Type VIIb secretion systems (T7SSb) were recently proposed to mediate different aspects of Firmicutes physiology, including bacterial pathogenicity and competition. By systematically investigating protein-protein interactions, we reveal that the membrane subunit YukC contacts all T7SSb components, including the WXG100 substrate YukE and the LXG effector YxiD. Taken together, these results provide a comprehensive picture of the network of T7SSb subunit interactions and identify YukC as their interaction hub. Altogether, our results suggest that pseudokinases have three key roles in the T7SSb secretion mechanism: substrate recruitment (LXG and WXG effectors), energy coupling (based on the cytoplasmic interaction with the ATPase, the dissociation-prone PK dimer, and the flexible β-swap region), and signal transduction (through the transmembrane stalk interacting with the putative pore-forming subunit).

We therefore produced a YukC413 construct lacking these residues, which promptly crystallized. In the crystal, YukC organized as a pseudosymmetrical dimer with chains A and B revolving around a virtual central axis (384 and 377 residues assigned, respectively). The YukC structure can be subdivided into four main regions from the N to the C terminus: the pseudokinase domain (residues 3 to 206), the β-swap domain (residues 207 to 211), the transmembrane (TM) domain (residues 220 to 243), and the extracellular domain (residues 244 to 384). The YukC structure reveals two unexpected features: a β-swap domain and a twisting stalk. Analysis of the dimer’s interfaces on the PDBe PISA web tool shows that YukC dimerization is mainly governed by the intermolecular interactions occurring within the stalk (solvation free energy gain upon formation of the interface [ΔiG] = −22), including the TM domain. The β-swap is located below the membrane plane, where the monomers cross as antiparallel β-strands. The symmetry of the structure is broken at the level of the pseudokinase domains, which are oriented differently in the two monomers. Interestingly, in the YukC structure, the orientation of the monomers diverges below the β-swap. This asymmetry is related to the different orientations of helix α8 in the two PK domains, favoring the H-bond between residues K205 of chain A and A80 of chain B (red asterisk). As a consequence, the PK domain of one monomer (chain B) is closer to the membrane plane than the other. Taken together, these sequence and structural analyses, as well as in vitro ATP-binding assays, suggest that YukC is unable to bind ATP (and to hydrolyze it).

>[2x]MSGEQKSYLENQLEAVAEKTDAGYTFTFQREKIKLLDGLEANVIKDINPFFHKEIDVTDDEVIITIQPPSSYKAFRFMKAKDKKSKWQFAYQLVQAVQQHNLSRLNLIVAPENIVFDKGLTPYFLHYGVKESIPPYERDEERVWQELKAAAALAVDGAFAFEDYLKFNETLTFSAEAKAILDAESYDDLLELIQTHIDELEAKAKTYIHIPRKKWNIQRYIGLGLIVLLVPALIYSMYALFFAQPKHQAIVDSNRAFLNKQYSEVISTLSKYDAESLPESVQYQLATSYVEVENLGSAKTKNIENNLVTLQSDPQHFLYWIDYGRGEYKEAISIGRKLEYNDYIYFALAKYKQQLLSEDTNDEDIQKELDSVNSELEKAQKERQENKQSNSETSLVDTSEEQTQTDEEKQAEEWSHPQFEKAA>[2x]SDQDYRARLVYPFSGAISPHADIVDQATLAWAAMFGLLTDSLRHKSRRLQYGLLAARAYPRADREMLQIAADWIAWLFFMDDQCDETGIGRDLQRMIALHERFLAILDGATPEAHDC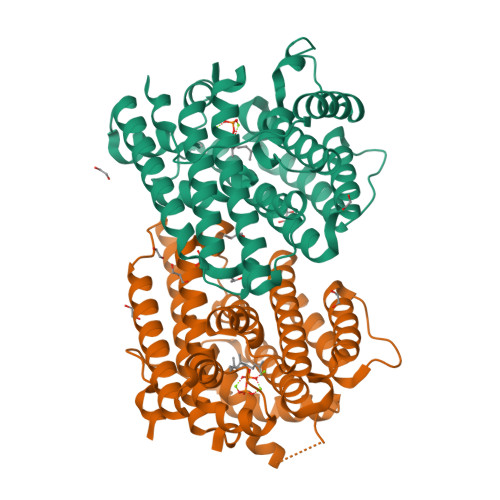ALTYALADLRRRLALRAPDNWLRRFSEHVRLYFTANRWETVNRQRGATPNVATYCAARLFSGAVYACFDLIELAEQIELPFYARHHSIVQQLEQAANNIICWCNDVLSYPKEMQHGDRHNLVLVIQGEHQCSLPEAIDRALDLHAREVATFVRKRTCVPYFDAAVNTALEKYVTGLQFWICANRDWSLTATRYA> MKLTLDITDWQAIAPGLSLTEEWKAWSATLPAAIDKSRPLEKCTQLPMMTARRLSSGSRLAVDCGLSLLRRHQVDAIVYTSRHGELERNYQILQNLAQQESISPTNFAMSVHNSSVGNLTIVAKAPLVSSSVSAGIDS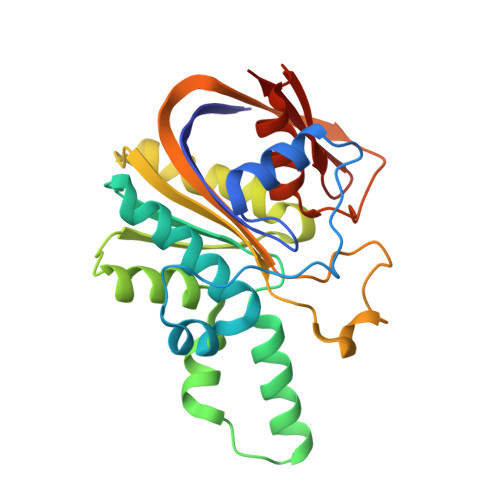FQQGLFEALTLIHAGHRKVLFVDFEGEIPGFYHNVIDAKTPTYPFAVALLLEQGAGLSCTKQSSMETEPSLPQSLQFLHGWLRGEQHFVVSGDHCQWNWSR> MLAKRIIACLDVKDGRVVKGSNAENLRDSGDPVELGKFYSEIGIDELVFLDITASVEKRKTMLELVEKVAEQIDIPFTVGGGIHDFETASELILRGA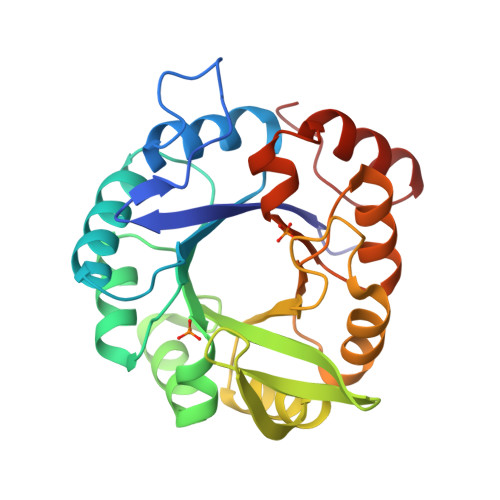DKVSINTAAVENPSLITQIAQTFGSQAVVVAIDAKRVDGEFMVFTYSGKKNTGILLRDWVVEVEKRGAGEILLTSIDRDGTKSGYDTEMIRFVRPLTTLPIIASGGAGKMEHFLEAFLAGADAALAASVFHFREIDVRELKEYLKKHGVNVRLEGL> GSGFTSKDTYLSHFNPRDYLEKYYKFGSRHSAESQILKHLLKNLFKIFCLDGVKGDLLIDIGSGPTIYQLLSACESFKEIVVTDYSDQNLQELEKWLKKEPAAFDWSPVVTYVCDLEGNRVKGPEKEEKLRQAVKQVLKCDVTQSQPLGAVPLPPADCVLSTLCLDAACPDLPTYCRALRNLGSLLKPGGFLVIMDALKGGGGREAVEAAVKEAGYTIEWFEVIS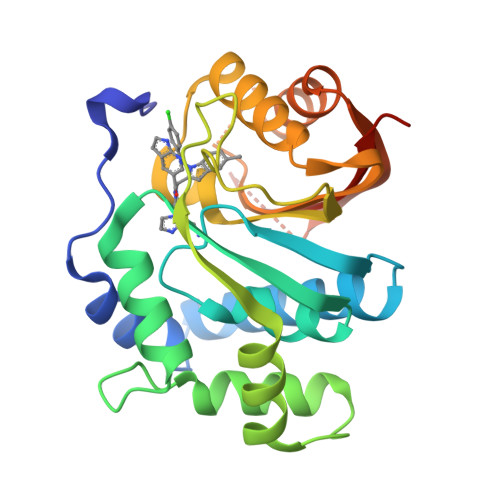QSYSSTMANNEGLFSLVARKLSRPL The major facilitator superfamily (MFS) glucose transporter GLUT4 mediates the rate-limiting glucose cellular uptake in adipocytes and muscle cells, and thus plays a vital role in insulin-responsive glucose metabolism. At basal state, GLUT4 is primarily distributed on the membranes of the trans-Golgi network (TGN), endosomes and 50–70 nm tubulo-vesicular structures known as the GLUT4 storage vesicles (GSVs). Upon insulin stimulation, GLUT4 is quickly transported from these intracellular structures to the plasma membrane, resulting in rapid consumption of glucose from blood. Among the SLC2A members, GLUT4 is most closely related to GLUT1, with a sequence identity and similarity of 65% and 79%, respectively.

We also successfully reconstituted the purified GLUT4 into nanodiscs of POPC plus cholesterol surrounded by the membrane scaffold protein MSP1D1. The elution volume of nanodisc-embedded GLUT4 is slightly earlier than β-NG. To stabilize the structure of GLUT4, 1 mM CCB was added to the purified proteins. Following our previously developed “guided multi-reference 3D classification” and “seed”-facilitated 3D classification strategy, the resolutions of GLUT4 embedded in the LMNG/CHS micelles and nanodiscs both reached 3.3 Å after several rounds of 3D classification and refinement by cryoSPARC. In the structure of GLUT4, the amino terminal domain (NTD, containing TMs 1-6) and carboxyl terminal domain (CTD, containing TMs 7-12) enclose a large cavity that opens to the intracellular side, a state defined as inward-open (left). CCB is accommodated in the big cleft between the NTD and CTD. The macrolide ring of CCB is coordinated by Asn176 and Trp404 through polar interactions, and Phe38, Trp404, and Trp428 through hydrophobic interaction. In the cryo-EM map for GLUT4, a characteristic glycan density is observed contiguous with Asn57, exemplifying the unique power of cryo-EM in resolving posttranslational modifications. The major distinction occurs to ICH5, which is invisible in the structure of GLUT1, but clearly resolved in the EM map of GLUT4. None of the GLUT4-unique sequences, 5FQQI8, 489LL490, and 498TELEY502, is visible, likely owing to the intrinsic flexibility of these segments.

> MDYKDDDDKGTMPSGFQQIGSEDGEPPQQRVTGTLVLAVFSAVLGSLQFGYNIGVINAPQKVIEQSYNETWLGRQGPEGPSSIPPGTLTTLWALSVAIFSVGGMISSFLIGIISQWLGRKRAMLVNNVLAVLGGSLMGLANAAASYEMLILGRFLIGAYSGLTSGLVPMYVGEIAPTHLRGALGTLNQLAIVIGILIAQVLGLESLLGTASLWPLLLGLTVLPALLQLVLLPFCPESPRYLYIIQNLEGPARKSLKRLTGWADVSGVLAELKDEKRKLERERPLSLLQLLGSRTHRQPLIIAVVLQLSQQLSGINAVFYYSTSIFETAGVGQPAYATIGAGVVNTVFTLVSVLLVERAGRRTLHLLGLAGMCGCAILMTVALLLLERVPAMSYVSIVAIFGFVAFFEIGPGPIPWFIVAELFSQGPRPAAMAVAGFSNWTSNFIIGMGFQYVAEAMGPYVFLLFAVLLLGFFIFTFLRVPETRGRTFDQISAAFHRTPSLLEQEVKPSTELEYLGPDEND>[2x]GAFMSSGPRLNTDYTSANQDSRVQFIVLHYTSTDLPHSLGILTHGGVSAHYLIGDDEPATVYRLVDENRRAWHAGVSEWQGRTWLNATSIGIEIVNQGY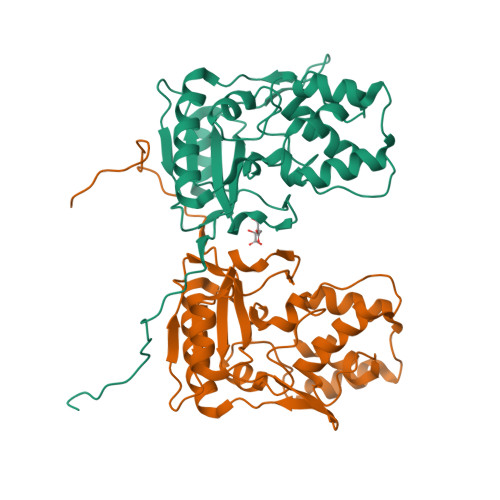RDTPQGRVWYPFSEAQIQALIPLLKDIAKRHGITPDRIIGHSDIAPGRKVDPGPLFPWKRLADAGLVPWPKPGELARRLAELNGQLPDVRWFQQQLARHGYLVPQTGELEKDTRDVIGAFQMKYRPARFDGEPDLETAALLLAVPTS>MASMTGGQQMGRGSEFMIASVRGEVLEVALDHVVIEAAGVGYRVNATPATLATLRQGTEARLITAMIVREDSMTLYGFPDGETRDLFLTLLSVSGVGPRLAMAALAVHDAPALRQVLADGNVAALTRVPGIG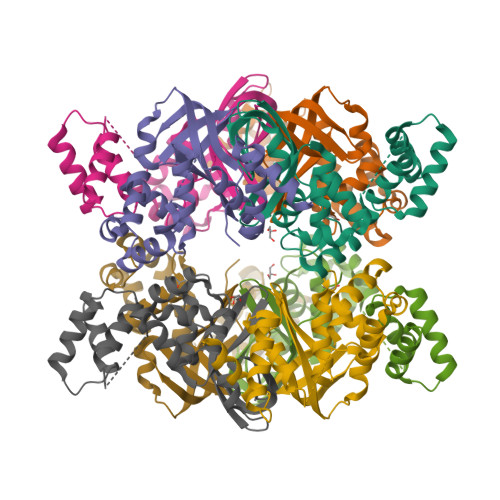KRGAERMVLELRDKVGVAATGGALSTNGHAVRSPVVEALVGLGFAAKQAEEATDTVLAANHDATTSSALRSALSLLGKAR[4x]> GSMTEIALIGNPNSGKTSLFNLITGHNQRVGNWPGVTVERKSGLVKKNKDLEIQDLPGIYSMSPYSPEAKVARDYLLSQRADSILNVV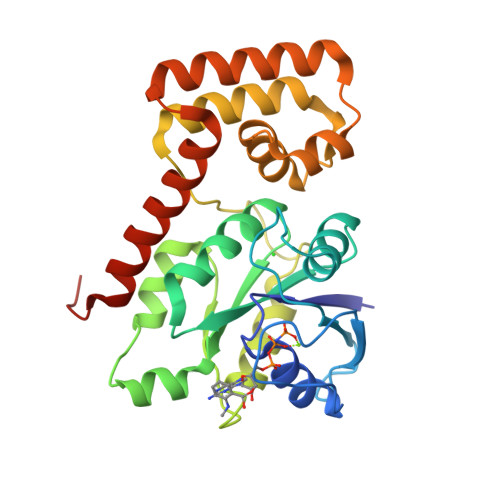DATNLERNLYLTTQLIETGIPVTIALNMIDVLDGQGKKINVDKLSYHLGVPVVATSALKQTGVDQVVKKAAHTTTSTVGDLAFPIYDDRLEAAISQILEVLGNSVPQRSARFYAIKLFEQDSLVEAELDLSQFQRKEIEDIIRITEEIFTEDAESIVINERYAFIERVCQMAESHTEDFALTLS>MAPSLDSISHSFANGVASAKQAVNGASTNLAVAGSHLPTTQVTQVDIVEKMLAAPTDSTLELDGYSLNLGDVVSAARKGRPVRVKDSDEIRSKIDKSVEFLRSQLS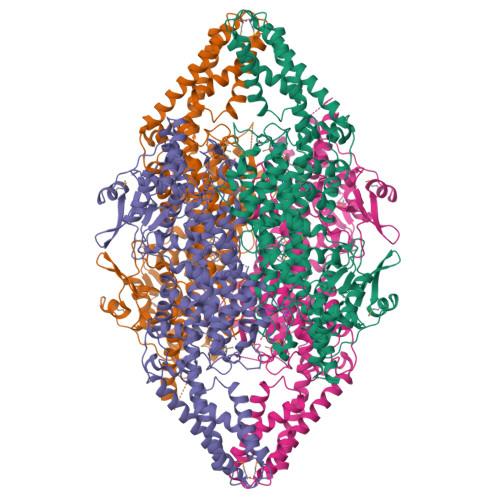MSVYGVTTGFGGSADTRTEDAISLQKALLEHQLCGVLPSSFDSFRLGRGLENSLPLEVVRGAMTIRVNSLTRGHSAVRLVVLEALTNFLNHGITPIVPLRGTISASGDLSPLSYIAAAISGHPDSKVHVVHEGKEKILYAREAMALFNLEPVVLGPKEGLGLVNGTAVSASMATLALHDAHMLSLLSQSLTAMTVEAMVGHAGSFHPFLHDVTRPHPTQIEVAGNIRKLLEGSRFAVHHEEEVKVKDDEGILRQDRYPLRTSPQWLGPLVSDLIHAHAVLTIEAGQSTTDNPLIDVENKTSHHGGNFQAAAVANTMEKTRLGLAQIGKLNFTQLTEMLNAGMNRGLPSCLAAEDPSLSYHCKGLDIAAAAYTSELGHLANPVTTHVQPAEMANQAVNSLALISARRTTESNDVLSLLLATHLYCVLQAIDLRAIEFEFKKQFGPAIVSLIDQHFGSAMTGSNLRDELVEKVNKTLAKRLEQTNSYDLVPRWHDAFSFAAGTVVEVLSSTSLSLAAVNAWKVAAAESAISLTRQVRETFWSAASTSSPALSYLSPRTQILYAFVREELGVKARRGDVFLGKQEVTIGSNVSKIYEAIKSGRINNVLLKMLA[8x]> MASGLYLFVMNIRSVFKLDELGSEVLRIAVPASLALAADPLASLVDTAFIGHLGSVEIAAVGVSIAIFNQVSKVCIYPLVSVTTSFVAEEDAIISKYLEEKKRYIPSVTSALIVGSFLGLVQAVFLIFSAKFVLGIMGVKHDSPMLEPAVRYLTIRSLGAPAVLLSLAMQGVFRGFKDTKTPLYATVVGDATNIILDPILMFVCHMGVTGAAVAHVISQYLITMILICRLVQQVDVIPPSLKSLKFGRFLGAGFLLLARVVAVTFCVTLASSLAARDGPTIMAAFQICLQLWLATSLLADGLAVAGQAVLASAFAKNDHKKVIAATSRVLQLSIVLGMGLTVVLGLFMKFGAGVFTSDADVINVIHKGIPFVAGTQTINALAFVFDGINFGAQDYVYSAYSMVGVASISIPCLVYLSAHKGFIGIWV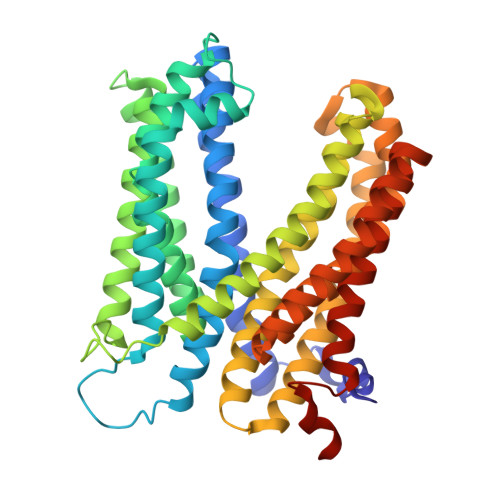ALTIYMSLRTVASTWRMGAARGPWVFLRKAGGENLYFQ>HHHHHHPCCSNPCQNRGECMSTGFDQYKCDCTRTGFYGENCTTPEFLTRIKLLLKPTPNTVHYILTHFKGVWNIVNNIPFLRSLIMKYVLTSRSYLIDSPPTYNVHYGYKSWEAFSNLSYYTRALPPVADDCPTPMGVKGNKELPDSKEVLEKVLLRREFIPDPQGSNMMFAFFAQHFTHQFFKTDHKRGPGFTRGLGHGVDLNHIYGETLDRQHKLRLFKDGKLKYQVIGGEVYPPTVKDTQVEMIYPPHIPENLQFAVGQEVFGLVPGLMMYATIWLREHNRVCDILKQEHPEWGDEQLFQTSRLILIGETIKIVIEDYVQHLSGYHFKLKFDPELLFNQQFQYQNRIASEFNTLYHWHPLLPDTFNIEDQEYSFKQFLYNNSILLEHGLTQFVESFTRQIAGRVAGGRNVPIAVQAVAKASIDQSREMKYQSLNEYRKRFSLKPYTSFEELTGEKEMAAELKALYSDIDVMELYPALLVEKPRPDAIFGETMVELGAPFSFKGLMGNPICSPQYWKPSTFGGEVGFKIINTASIQSLICNNVKGCPFTSFNVQDP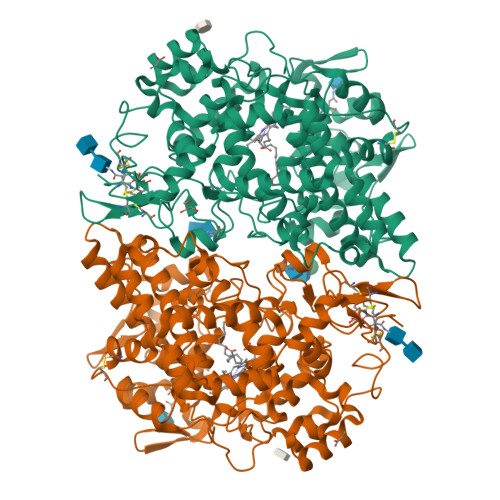QPTKTATIAASASHSRLDDINPTVLIKRRSTEL[2x]>GQSGPLPKPSLQALPSSLVPLEKPVTLRCQGPPGVDLYRLEKLSSSRYQDQAVLFIP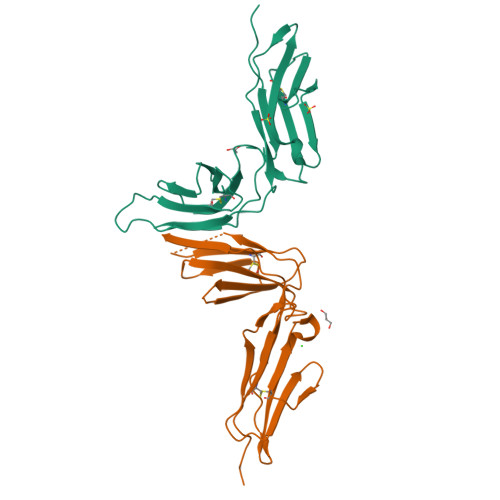AMKRSLAGRYRCSYQNGSLWSLPSDQLELVATGVFAKPSLSAQPGPAVSSGGDVTLQCQTRYGFDQFALYKEGDPAPYKNPERWYRASFPIITVTAAHSGTYRCYSFSSRDPYLWSAPSDPLELVVT[2x]> YDYFQFTQQYQLAVCNSNRTLCKDPPDKLFTVHGLWPSNMVGPDPSKCPIKNIRKREKLLEHQLEIIWPNVFDRTKNNLFWDKEWMKHGSCGYPTIDNENHYFETVIKMYISKKQNVSRILSKAKIEPDGKKRALLDIENAIRNGADNKKPKLKCQKKGTTTELVEITLCSDKSGEHFIDCPHPFEPISPHYCPTNN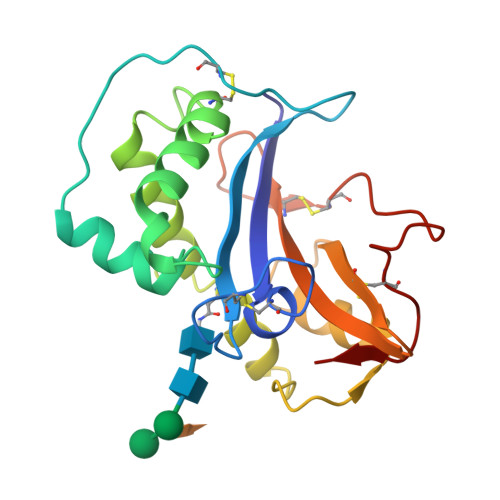IKY> MRYIRLCIISLLATLPLAVHASPQPLEQIKLSESQLSG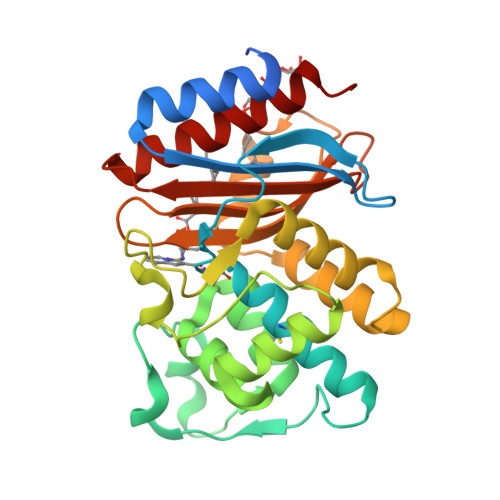RVGMIEMDLASGRTLTAWRADERFPMMSTFKVVLCGAVLARVDAGDEQLERKIHYRQQDLVDYSPVSEKHLADGMTVGELCAAAITMSDNSAANLLLATVGGPAGLTAFLRQIGDNVTRLDRWETELNEALPGDARDTTTPASMAATLRKLLTSQRLSARSQRQLLQWMVDDRVAGPLIRSVLPAGWFIADKTGAGERGARGIVALLGPNNKAERIVVIYLRDTPASMAERNQQIAGIGAALIEHWQR>[2x]DSNGNQEINGKEKLSVNDSKLKDFGKTVPVGIDEENGMIKVSFMLTAQF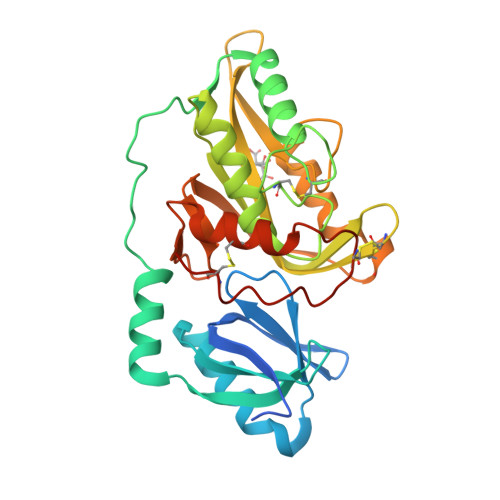YEIKPTKENEQYIGMLRQAVKNESPVHIFLKPNSNEIGKVESASPEDVRYFKTILTKEVKGQTNKLASVIPDVATLNSLFNQIKNQSCGTSTASSPCITFRYPVDGCYARAHKMRQILMNNGYDCEKQFVYGNLKASTGTCCVAWSYHVAILVSYKNASGVTEKRIIDPSLFSSGPVTDTAWRNACVNTSCGSASVSSYANTAGNVYYRSPSNSYLYDNNLINTNCVLTKFSLLSGCSPSPAPDVSSCGFHHHHHH>MSNPYERGPAPTESSVTAVRGYFDTDTDTVSSLVSGFGGGTIYYPTDTSEGTFGGVVIAPGYTASQSSMAWMGHRIASQGFVVF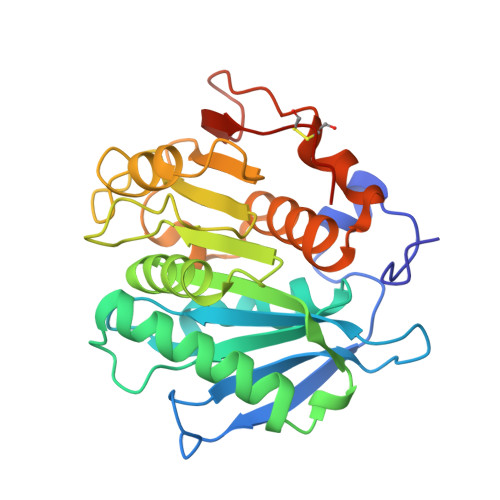TIDTITRYDQPDSRGRQIEAALDYLVEDSDVADRVDGNRLAVMGHSMGGGGTLAAAENRPELRAAIPLTPWHLQKNWSDVEVPTMIIGAENDTVASVRTHSIPFYESLDEDLERAYLELDGASHFAPNISNTVIAKYSISWLKRFVDEDERYEQFLCPPPDTGLFSDFSDYRDSCPHTTLEHHHHHH[2x]2-(4-{[1-(4-CHLOROBENZYL)PIPERIDIN-4-YL]METHOXY}PHENYL)-1H-BENZIMIDAZOLE-5-CARBOXAMIDE 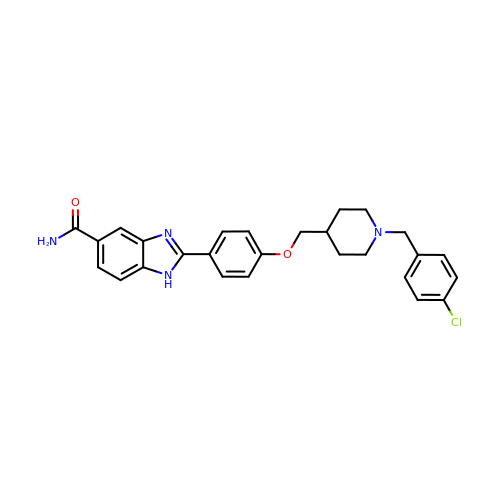| C27 H27 Cl N4 O2 | LKKIDFQBVDANKO-UHFFFAOYSA-N>[2x]MNSTPKGTIYLTFDDGPVNASVEVIKVLNQGGVKATFYFNAWHLDGIGDENEDRALEALKLALDSGHIVGNHSYDHMIHNCVEEFGPTSGADCNATGNHQIHSYQDPVR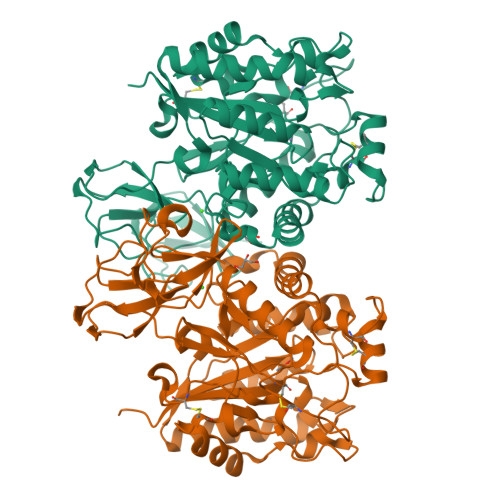DAASFEQNLITLEKYLPTIRSYPNYKGYELARLPYTNGWRVTKHFQADGLCATSDNLKPWEPGYVCDPANPSNSVKASIQVQNILANQGYQTHGWDVDWAPENWGIPMPANSLTEAVPFLAYVDKALNSCSPTTIEPINSKTQEFPCGTPLHADKVIVLTHDFLFEDGKRGMGATQNLPKLAEFIRIAKEAGYVFDTMDNYTPRWSVGKTYQAGEYVLYQGVVYKAVISHTAQQDWAPSSTSSLWTNADPATNWTLNVSYEQGDIVNYKGKRYLVSVPHVSQQDWTPDTQNTLFTALELRRQWSHPQFEK> LGQEKERFQVLPGRDKMLYVAAQNERDTLWARQVLARGDYDKNARVINENEENKRISIWLDTYYPQLAYYRIHFDEPRKPVFW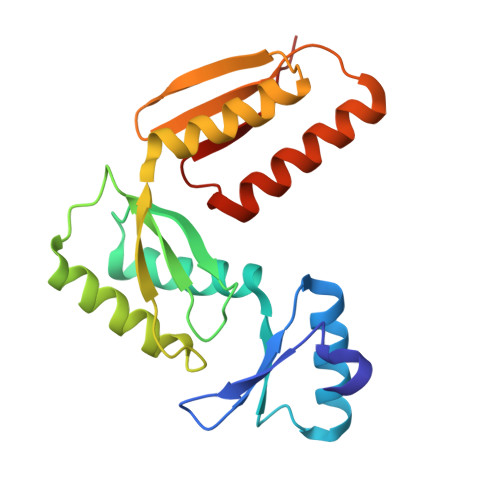LSRQRNTMSKKELEVLSQKLRALMPYADSVNITLMDDVTAAGQAEAGLKQQALPYSRRNHKGGVTFVIQGALDDVEILRARQFVDSYYRTWGGRYVQFAIELK In previous work we have explored the potential for establishing a bump-&-hole system targeting the bromodomains of the BET (bromo and extra-terminal) protein family. These four human proteins – BRD2, BRD3, BRD4 and BRDT – each contain two tandem bromodomains that bind acetylated lysine residues in histone tails, leading to the recruitment of multi-protein complexes to chromatin. Through this function the BET proteins play a significant role in controlling transcription and regulating gene expression. The phenotypes generated by said inhibitors have been used to investigate the functions of BET proteins and their significance as therapeutic targets. This process has been limited by the pan-selective nature of the BET inhibitors, as they typically target all BET bromodomains with similar potency, hence specific proteins/bromodomains cannot be associated to specific phenotypes. Through structural analysis of the bromodomain we hypothesized that a leucine/valine substitution (L/V) would be a more conservative change than the previous L/A substitution, resulting in a smaller ‘hole’ but still allowing enough space to accommodate a bumped ligand.

We used isothermal titration calorimetry (ITC) to measure the affinity and thermodynamic parameters for di-acetylated H4K(5,8)ac and tetra-acetylated H4K(5,8,12,16)ac substrate peptides12 binding to BET bromodomain constructs. The L/V mutation typically decreased the affinity of the peptide:bromodomain interaction by around two-fold (Table S2†), which is close to experimental errors and a significant improvement over the L/A mutation which showed up to 10-fold decreases in affinity. Analysis of the thermodynamic parameters of binding (ΔH, TΔS, ΔG) suggested that the L/V mutation does not substantially impact the binding mode of these peptides. The conformation of the ZA loop in the L/V mutant structure superposes very well with that of the WT (so-called “open” conformation), which differs from that observed in the L/A mutant, which is in a closed conformation. Re-orienting the ZA loop during binding might be contributing to the varying affinities observed between WT and mutant bromodomains for acetylated histone peptides. However, differences in crystallization space group and consequently crystal packing around the ZA loop amongst the various crystal structures might also contribute to the different conformations observed for the ZA loop.

> SMGKLSEQLKHCNGILKELLSKKHAAYAWPFYKPVDASALGVHDYHDIIKHPMDLSTVKRKMENRDYRDAQEFAADVRLMFSNCYKYNPPDHDVVAMARKLQDVFEFRYAKMPD> ANEGSKTLQRNRKMAMGRKKFNMDPKKGIQFLVENELLQNTPEEIARF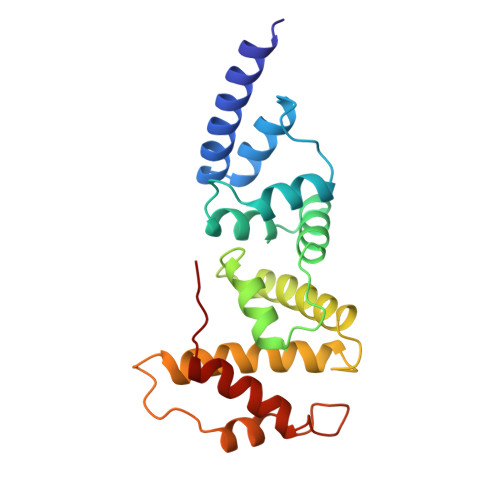LYKGEGLNKTAIGDYLGEREELNLAVLHAFVDLHEFTDLNLVQALRQFLWSFRLPGEAQKIDRMMEAFAQRYCLCNPGVFQSTDTCYVLSFAVIMLNTSLHNPNVRDKPGLERFVAMNRGINEGGDLPEELLRNLYDSIRNEPFKIP>[2x]GGUAUUGCGG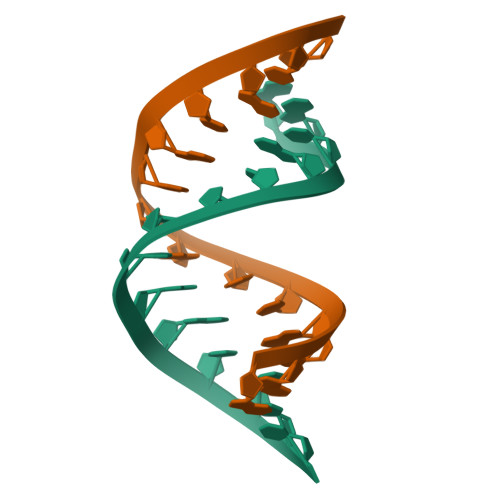UACC>[4x]MSNATLNQLPGRLGDPSMSLGTDPRTDPRLAAALTQLGLADQAAEPPVNANSEVADCIAYSTAAEQAWQTLFAMLGSQGEPSNPVDVREETIKG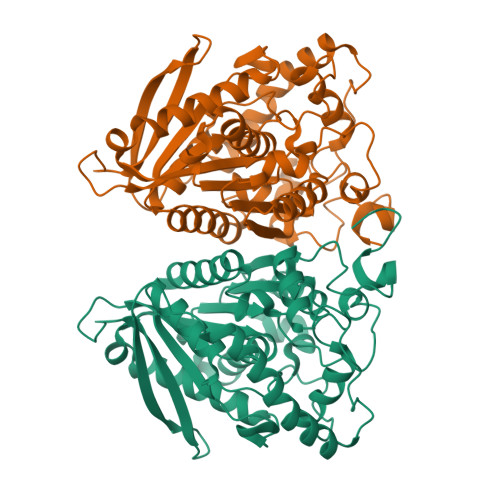RGGNEIKLYIHSPTGHTSDSDPLPCVVHTHGGGMVILTAADANYSRWRSELAATGLVVVGVEFRNAAGALGNHPFPAGLHDCADAAKWVASNREALGISTLIMSGESGGGNLSLATTMLAKKEGWLEEIAGVYAQCPYISGLYASKPEELPSLLENDAYFWDMKTMGAMVKPYDPTGENASNPLAWPYHASLEDLAGLPPHVISVNELDPLRDEGLAHYRKLLKAGVSTVGRTVHGTCHAADCSFVDVIPDVYFATVRDISAFAYSRA> MFQQLSARLQEAIGRLRGRGRITEEDLKATLREIRRALMDADVNLEVARDFVERVREEALGKQVLESLTPAEVILATVYEALKEALGGEARLPVLKDRNLWFLVGLQGSGKTTTAAKLALYYKGKGRRPLLVAADTQRPAAREQLRLLGEKVGVPVLEVMDGESPESIRRRVEEKARLEARDLILVDTAGRLQIDEPLMGELARLKEVLGPDEVLLVLDAMTGQEALSVARAFDEKVGVTGLVLTKLDGDARGGAALSARHVTGK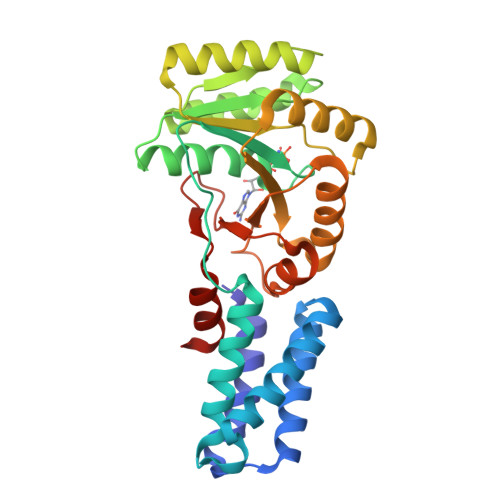PIYFAGVSEKPEGLEPFYPERLAGRILGMGD{1-[(5-chloro-2-methyl-1-benzothiophen-3-yl)methyl]-6-(3,5-diaminophenyl)-1H-indol-3-yl}acetic 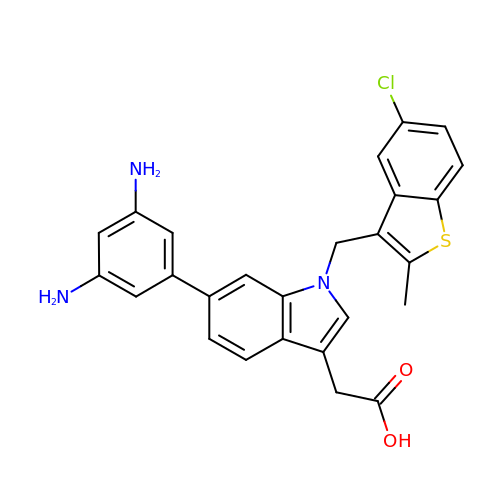acid | C26 H22 Cl N3 O2 S | PFDAXQGFXBAMGF-UHFFFAOYSA-N> QPIFLNVLEAIEPGVVCAGHDNNQPDSFAALLSSLNELGERQLVHVVKWAKALPGFRNLHVDDQMAVIQYSLMGLMVFAMGWRSFTNVNSAMLYFAPDLVFNEYRMHKSRMYSQCVRMRHLSQEFGWLQITPQEFLCMKALLLFSIIPVDGLKNQKFFDELRMNYIKELDRIIACKRKNPTSCSRRFYQLTKLLDSVQPIARELHQFTFDLLIKSHMVSVDFPEMMAEI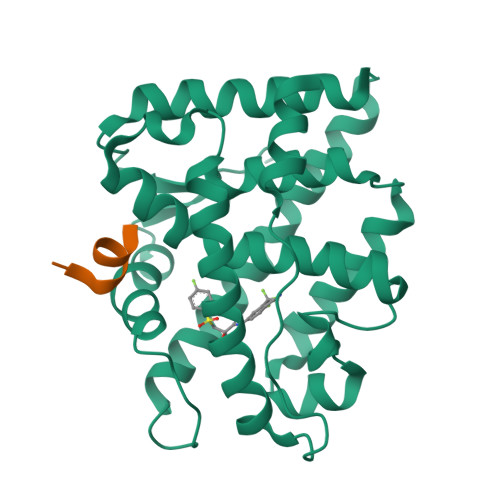ISVQVPKILSGKVKPIYFHTQ;> SDSAFSRYYTRS> PLAAGAVILRRFAFNAAEQLIRDINDVASQSPFRQMVTPGGYTMSVAMTNCGHLGWTTHRQGYLYSPIDPQTNK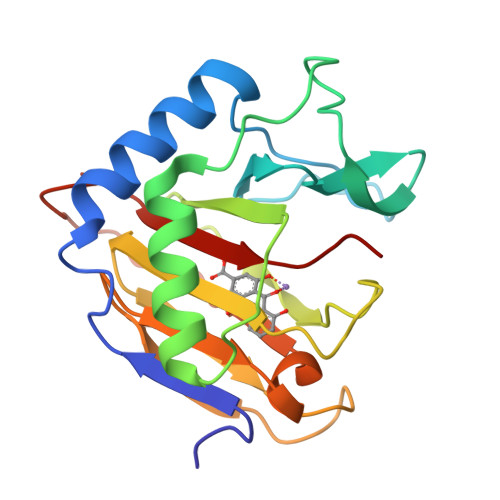PWPAMPQSFHNLCQRAATAAGYPDFQPDACLINRYAPGAKLSLHQDKDEPDLRAPIVSVSLGLPAIFQFGGLKRNDPLKRLLLEHGDVVVWGGESRLFYHGIQPLKAGFHPLTIDCRYNLTFRQAGKKE> EGPPKYTKSILKKGDKTNFPKKGDVVHCWYTGTLPDGTVFDTNIQTSSKKKKNAKPLSFKVGVGKVIRGWDEA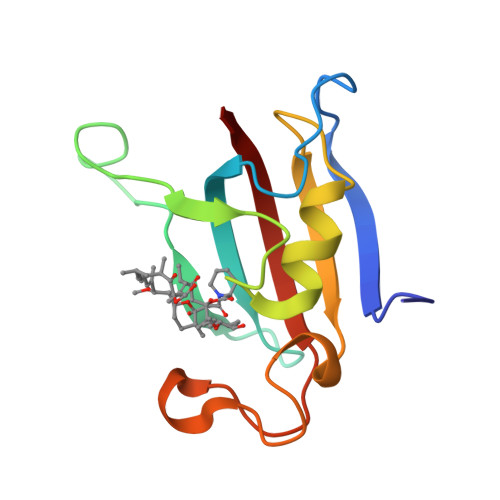LLTMSKGEKARLEIEPEWAYGKKGQPDAKIPPNTKLIFEVELVDID>[4x]RPFLPKKKQQKDSLINLKIQKENPKVVNEINIEDLSLTKAAYCRCWRSKTFPACDGSH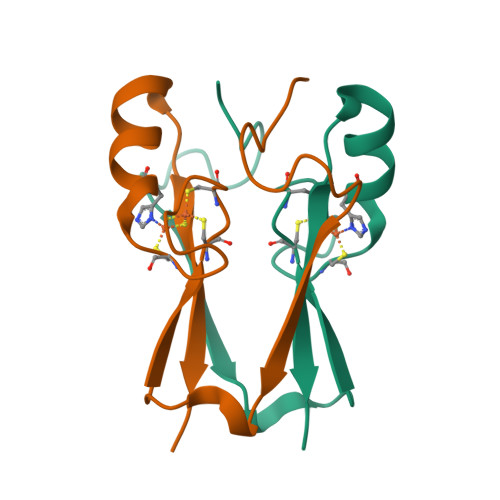NKHNELTGDNVGPLILKKKEV> MDLKAQSIPFAWLDRDKVQRLTNFLSNLENLENVDLREHPYVTNSCVVREGEDVDELKTLYNTFILWLMYHYVLSKRKPDYNAIWQDITKLQNVVNEYLKSKGLNKGNFENMFTNKEKFESQFSDIHRALLRLGNSIRWGSNVPIDTPYVNLTAEDSSEIENNLQDAEKNMLWYTVYNINDPWDENGYLVTSINKLVYLGKLFVTLNQSWSKLEKVAMSQIVTTQNHLSGHLRKNENFNAVYSQRVLQTPLTGQRVESFLKIITSDYEIIKSSLESYSASKAFSVPENGPHSLMDFASLDGRMPSDLSLPSISIDTKRPSADLARLKISQPKSLDAPLKTQRRHKFPESDSVDNAGGKILIKKETLGGRDVRATTPVSSVSLMSGVEPLSSLTSTNLDLRDKSHGNYRIGPSGILDFGVKLPAEAQSNTGDVDLLQDKTSIRSPSSGITDVVNGLANLNLRQNKSDVSRPWSKNTAANADVFDPVHRLVSEQTGTPFVLNNSDVAGSEAKLTTHSTETGVSPHNVSLIKDLRDKDGFRKQKKLDLLGSWTKEKNDKAIVHSREVTGDSGDATETVTARDSPVLRKTKHANDIFAGLNKKYARDVSRGGKGNSRDLYSGGNAEKKETSGKFNVDKEMTQNEQEPLPNLMEAARNAGEEQYVQAGLGQRVNKILAEFTNLISLGEKGIQDILHNQSGTELKLPTE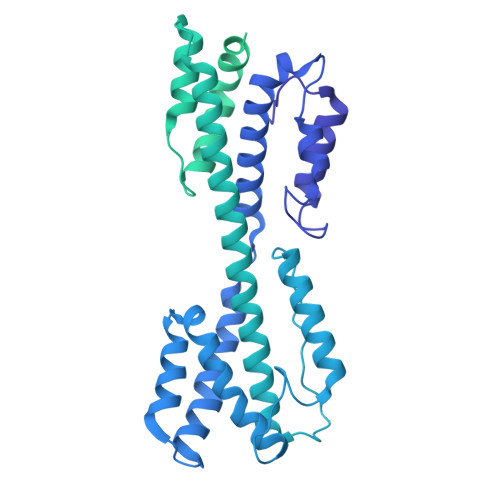NKLGRESEEANVERILEVSDPQNLFKNFKLQNDLDSVQSPFRLPNADLSRDLDSVSFKDALDVKLPGNGEREIDLALQKVKAGERETSDFKVGQDETLIPTQLMKVETPEEKDDVIEKMVLRIRQDGETDEETVPGPGVAESLGIAAKDKSVIAS>SNAMSVQVGVIMGSKSDWSTMKECCDILDNLGIGYECEVVSAHRTPDKMFDYAETAKERGL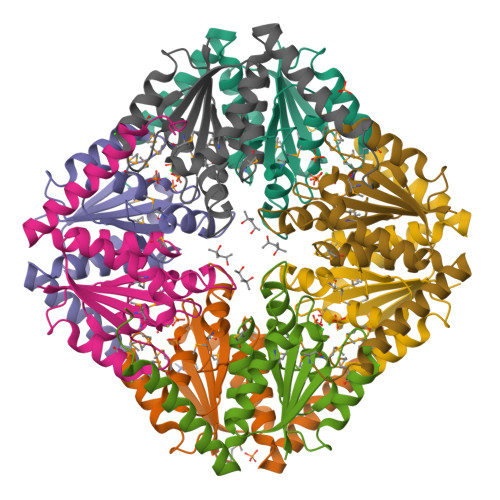KVIIAGAGGAAHLPGMVAAKTTLPVLGVPVKSSTLNGQDSLLSIVQMPAGIPVATFAIGMAGAKNAALFAASILQHTDINIAKALAEFRAEQTRFVLENPDPREH[8x]> AAVTQSPRNKVAVTGEKVTLSCQQTNNHNNMYWYRQDTGHGLRLIHYSYGAGSTEKGDIPDGYKASRPSQEQFSLILESATPSQTSVYFCASGGGGTLYFGAGTRLSVL;> ESQPDPM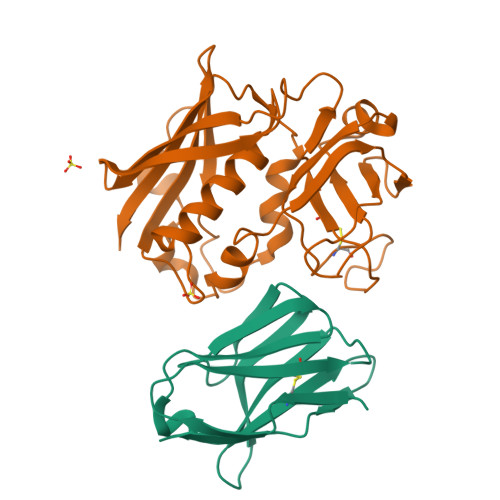PDDLHKSSEFTGTMGNMKYLYDDHYVSATKVKSVDKFLAHDLIYNISDKKLKNYDKVKTELLNEDLAKKYKDEVVDVYGSNYYVNCYFSSKDNVWWHGKTCMYGGITKHEGNHFDNGNLQNVLVRVYENKRNTISFEVQTDKKSVTAQELDIKARNFLINKKNLYEFNSSPYETGYIKFIENNGNTFWYDMMPAPGDKFDQSKYLMMYNDNKTVDSKSVKIEVHLTTKNG Cytohesins comprise a metazoan Arf GEF family with four mammalian paralogs (Grp1, ARNO, and cytohesins-1/4) that function in receptor signaling, endocytic trafficking, and cell adhesion/migration (Chardin et al., 1996, Fuss et al., 2006, Hafner et al., 2006, Hickman et al., 2018, Ito et al., 2018, Kolanus et al., 1996, Li et al., 2012, Mohanan et al., 2018, Ogasawara et al., 2000, Rafiq et al., 2017). All cytohesins share a common architecture comprised of a heptad repeat coiled coil (CC) domain, the Sec7 domain, and a pleckstrin-homology (PH) domain. The PH domain binds phosphatidyl inositol 3,4,5-trisphosphate (PIP3) and/or phosphatidyl inositol 4,5-bisphosphate (PIP2) (Chardin et al., 1996, Kavran et al., 1998, Klarlund et al., 1997), with affinities, specificities and spatiotemporal distributions dependent on splice variation in the phosphoinositide-binding pocket (Cronin et al., 2004, Klarlund et al., 2000, Ratcliffe et al., 2018). Two autoinhibitory elements, the Sec7-PH linker and C-terminal helix/polybasic region (CtH/PBR), strongly suppress GEF activity by occluding the active site in the Sec7 domain (DiNitto et al., 2007).

To address these issues and gain additional insight, the structural organization and extent of conformational variability of Grp114-399 dimers was independently investigated by single-particle NS-EM. Unsupervised reference-free classification of ∼10,000 manually picked particles from 500 micrographs yielded 53 good quality classes representing ∼6,500 particles. Attempts to generate a 3D reconstruction with visually selected particle classes were unsuccessful, suggesting potential conformational heterogeneity. To explore this possibility, the 2D class averages were systematically compared with 3D volume projections over the range of possible views for each model in the MultiFoXS pools. The 2D analysis suggested that conformational similarity of best scoring models might improve selection of classes for 3D reconstruction. For two class sets corresponding to compact or intermediate best scoring models, 3D volumes could be built and refined. Automated docking of the MultiFoXS pools with the refined 3D volumes selected best scoring models having relatively compact conformations similar to the more compact models in the six-state MultiFoXS ensembles. The low resolution of ∼53 Å for the refined 3D volumes likely reflects conformational heterogeneity in addition to negative staining. Flexibility in the CC-Sec7 linker is the main source of conformational variability, with a secondary contribution from hinge conformers that does not appear to be strongly influenced by dimerization. Although the analyses are most consistent with an antiparallel CC topology, the resolution is not sufficient to definitively exclude parallel or mixed topologies.

>[2x]MGHHHHHHGSPEDLSLEEREELLDIRRRKKELIDDIERLKYEIAEVMTEIDNLTSVEESKYTQRNAQIAMGRKKFNMDPKKGIQFLIENDLLQSSPEDVAQFLYKGEGLNKTVIGDYLGERDDFNIKVLQAFVELHEFADLNLVQALRQFLWSFRLPGEAQKIDRMMEAFASRYCLCNPGVFQSTDTCYVLSFAIIMLNTSLHNHNVRDKPTAERFITMNRGINEGGDLPEELLRNLYESIKNEPFKIPEDDGNDLTYTFFNPDREGWLLKLGGRVKTWKRRWFILTDNCLYYFEYTTDKEPRGIIPLENLSIREVEDPRKPNCFELYNPSHKGQVIKACKTEADGRVVEGNHVVYRISAPSPEEKEEWMKSIKASISRDPFYDMLATRKRRIANKK>[4x]TTLSCKVTSVEAITDTVYRVRIVPDAAFSFRAGQYLMVVMDERDKRPFSMASTPDEKGFIE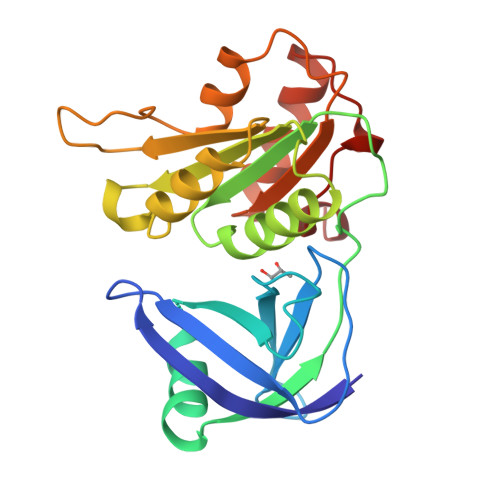LHIGASEINLYAKAVMDRILKDHQIVVDIPHGEAWLRDDEERPMILIAGGTGFSYARSILLTALARNPNRDITIYWGGREEQHLYDLCELEALSLKHPGLQVVPVVEQPEAGWRGRTGTVLTAVLQDHGTLAEHDIYIAGRFEMAKIARDLFCSERNAREDRLFGDAFAFI> GAQVSTQKTGAHE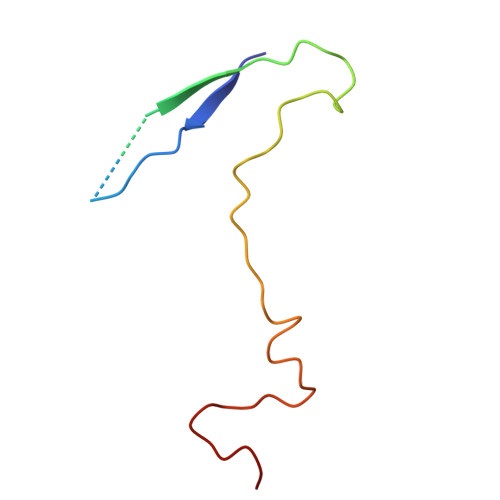TGLNASGNSIIHYTNINYYKDAASNSANRQDFTQDPGKFTEPVKDIMIKSLPALN P1-(5'-ADENOSYL)P5-(5'-THYMIDYL)PENTAPHOSPHATE 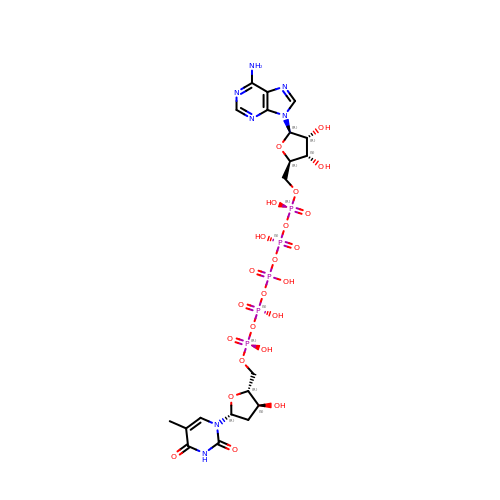| C20 H30 N7 O23 P5 | JCFDSPQTEMXXLO-SLFMBYJQSA-N> GAMDENDEGVRGTCEDASLCKRFAVSIGYWHDPYIQHFVRLSKERKAPEINRGYFARVHGVSQLIKAFLRKTECHCQIVNLGAGMDTTFWRLKDEDLLPSKYFEVDFPMIVTRKLHSIKCKPPLSSPILELHSEDTLQMDGHILDSKRYAVIGADLRDLSELEEKLKKCNMNTQLPTLLIAECVLVYMTPEQSANLLKWAANSFERAMFINYEQVNEGKSLESQKERLLSNGWETASAV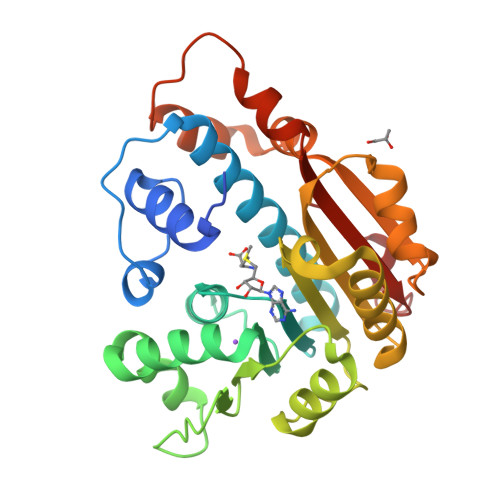DMMELYNRLPRAEVSRIESLEFLDEMELLEQLMRHYCLCWATKGGNELGLKEITY>[2x]GSGKAGVPGVAAPGAPAAAPPAKEIPEVLVDPRSRRRYVRGRFLGKGGFAKCFEISDADTKEVFAGKIVPKSLLLKPHQREKMSMEISIHRSLAHQHVVGFHGFFEDNDFVFVVLELCRRRSLLELHKRRKALTEPEARYYLRQIVLGCQYLHRNRVIHRDLKLGNLFLNEDLEVKIGDFGLATKVEYDGERKKTLCGTPNYIAPEVLSDAGHSFEVDVWSIGCIMYTLLVGKPPFET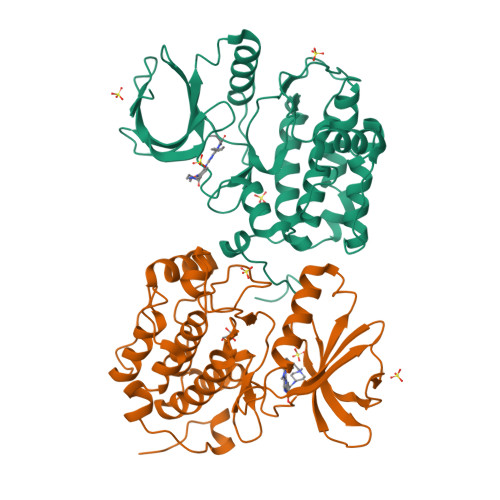SCLKETYLRIKKNEYSIPKHINPVAASLIQKMLQTDPTARPTINELLNDEFFTSGYIPARLPITCLTIPPRFSIAPSSLDPSNRKPL>MLANENSLLTMFRELGSGKLPLQIEQFERGKTIFFPGDPAERVYLLVKGAVKLSRVYESGEEITVALLRENSVFGVLSLLTGQRSDRFYHAVAFTPVQLFSVPIEFMQKALIERPELANVMLQGLSSRILQTEMMIETLAHRDMGSRLVSFLLILCRDFGIPSPDGITIDLKLSHQAIAEAIGSTRVTVTRLLGDLRESKLIAIHKKRITVFNPVALSQQFS[2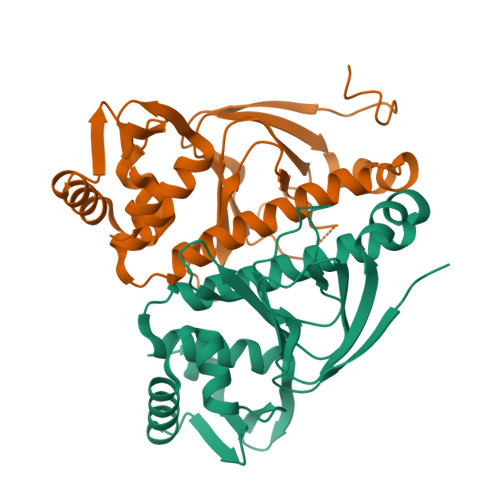x]>[2x]GIPLTPLFSRYKDSYLLYSFRLIDLLRASKSTHLTKLLSSQATYLYHFACLMKYKDIQKYEVQQLIEWAINASPDMDLQQFRIEFMDKTTELNLRSCQPKSFTYTFTTIWDTMHFLSLIIDDMVYTRDKSSLDFVMQQLKTMKVLFYNVFFILQCAMCRDHYMNVKGFIIYHIELIEIALDKEKYGTDITFVDSYQQETAGADVAVV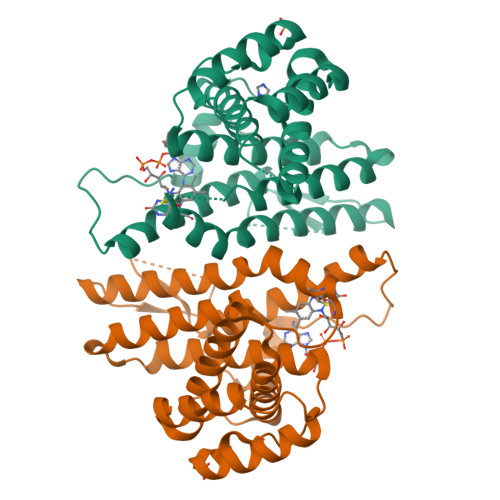SNNMLMKNLMAYVSMTFHNHINDYKWIQRNKKPPAHYERMTWGEYKKLLNLQL>[2x]SQSTRKKSRRNKWHFGVRCRGDAPEILLAVYRALQRAGAQFTVPKPVNGKYRSDMYTIKSRWEIPHCKREGKNTYAYIELQLYEVMPGCFMLDVKSNGYKDIYSHPERTADHGMDDLKSSFPFLDLCAMLVCKLFSA;>[2x]MSESEQYSTEIPAFLTSNTLQELKLPKPPSLPPHLEKCILNSNTAYKEDQSVLPNPNHVLLNHLAAANTQLGVLALSATTR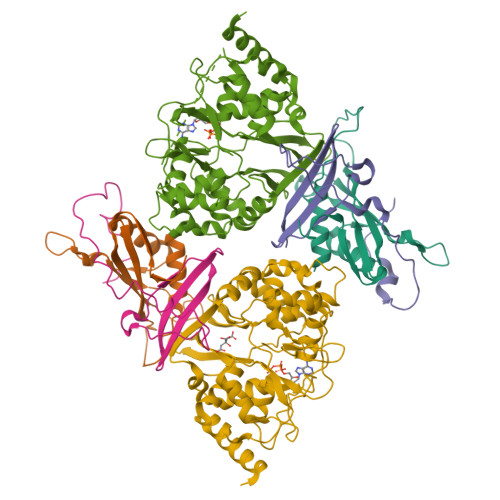YHRKYVTTAMFKNFDV;>[2x]MDVQETQKGALKEIQAFIRSRTSYDVLPTSFRLIVFDVTLFVKTSLSLLTLNNIVSAPLWDSEANKFAGLLTMADFVNVIKYYYQSSSFPEAIAEIDKFRLLGLREVERKIGAIPPETIYVHPMHSLMDACLAMSKSRARRIPLIDVDGETGSEMIVSVLTQYRILKFISMNCKETAMLRVPLNQMTIGTWSNLATASMETKVYDVIKMLAEKNISAVPIVNSEGTLLNVYESVDVMHLIQDGDYSNLDLSVGEALLKRPANFDGVHTCRATDRLDGIFDAIKHSRVHRLFVVDENLKLEGILSLADILNYIIYDKTTTPGVPEQTDNFESAV The pathogenicity of Shigella sp. is dependent on a complex macromolecular machine, the type 3 secretion system (T3SS), that delivers into host cells a set of effector proteins required for invasion. Blockage of effector secretion before host cell contact is mediated, in part, by a protein that has been proposed to act as either a physical impediment to the entrance to the secretion apparatus, or as a gatekeeper that determines substrate hierarchy. Across bacterial species, this protein (known as MxiC in Shigella sp.) possesses only weak sequence homology and in some species exists as two separate polypeptide chains (e.g., in Yersinia sp. the homologue consists of YopN and TyeA). MxiC is an elongated rod-shaped molecule with a long axis of 86 Å.

In order to improve the quality of MxiC crystals, a shortened construct encompassing residues 74–355 (MxiCNΔ73) was expressed, purified and subjected to crystallization trials. Reductive methylation of MxiCNΔ73 yielded crystals that diffracted to higher resolution: 2.85 Å and 2.5 Å in space groups P212121 and P222, respectively. The first and last domains consist only of the X-bundle motif while the central domain also possesses a bent helix (α5) that is packed against domain 1. It is the first two domains of MxiC that are equivalent to YopN while the third domain of MxiC, equivalent to TyeA, is connected to domain 2 via a ten-residue linker. There are a total of seven independent MxiC molecules in the crystallographic asymmetric units of the three refined crystal forms. These structures reveal that, although the fold of each domain is maintained in all structures (rmsd over Cα atoms of domains 1, 2 and 3 are 0.5 Å, 0.9 Å and 0.8 Å, respectively), there is some flexibility at the interfaces between domains resulting in a “wobble” of the terminal domains about the central domain (rmsd over all Cα atoms of 1.4 Å). Interestingly, mapping of sequence conservation onto the structure across the more closely related Salmonella, Burkholderia and Shigella species reveals a hydrophobic patch on the surface of the central domain consisting of residues Leu222, Met226, Gly239, Leu242 and Leu245 (red circle). This region is buried by crystal contacts in all seven independent molecules of MxiC in the P212121, P222 and P43212 crystal forms, suggesting that this region may be a “hot spot” for protein–protein interactions. Surprisingly, the most striking difference instead involves the long á-helix (α9) in the central domain of MxiC, which is straight in all of our MxiC structures, but possesses a sharp kink in YopN when complexed with TyeA. As the sequence at the hinge is not conserved, and all MxiC molecules possess the straight helix conformation, these structures may represent genuine differences between species.

>[3x]HSSGLVPRGSHMSQERILDGEEDEINHKIFDLKRTLKDNLPLDRDFIDRLKRYFKDPSDQVLALRELLNEKDLTAEQVELLTKIINEIISGSEKSVNAGINSAIQAKLFGNKMKLEPQLLRACYRGFIMGNISTTDQYIEWLGNFGFNHRHTIVNFVEQSLIVDMDSEKPSCNAYEFGFVLSKLIAIKMIRTSDVIFMKKLESSSLLKDGSLSAEQLLLTLLYIFQYPSESEQILTSVIEVSRASHEDSVVYQTYLSSVNESPHDIFKSESEREIAINILRELVTSAYKKELSR> KRKRKR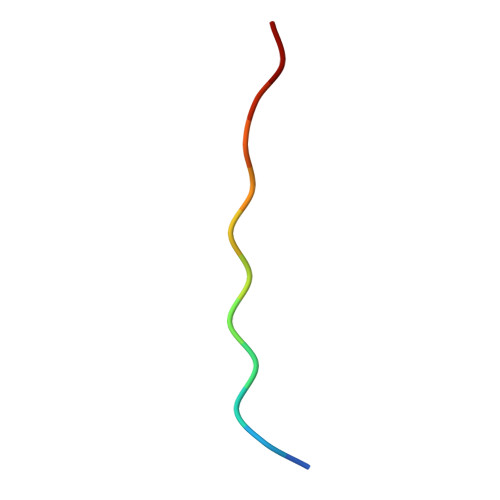KRKLSF> MHHHHHHLPNITILATGGTIAGGGDSATKSNYTVGKVGVENLVNAVPQLKDIANVKGEQVVNIGSQDMNDNVWLTLAKKINTDCDKTDGFVITHGTDTMEETAYFLDLTVKCDKPVVMVGAMRPSTSMSADGPFNLYNAVVTAADKASANRGVLVVMNDTVLDGRDVTKTNTTDVATFKSVNYGPLGYIHNGKIDYQRTPARKHTSDTPFDVSKLNELPKVGIVYNYANASDLPAKALVDAGYDGIVSAGVGNGNLYKSVFDTLATAAKTGTAVVRSSRVPTGATTQ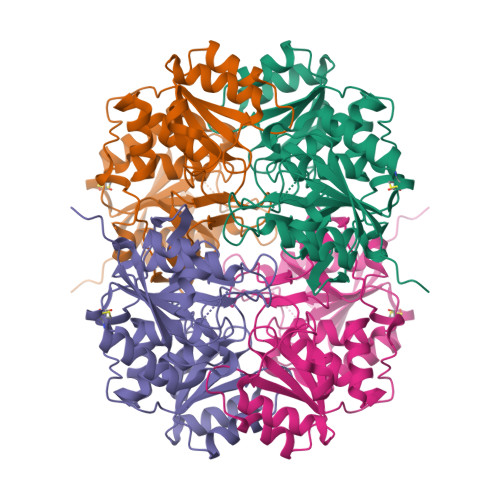DAEVDDAKYGFVASGTLNPQKARVLLQLALTQTKDPQQIQQIFNQY> ANIVGGIEYSINNASLCSVGFSVTRGATKGFVTAGHCGTVNATARIGGAVVGTFAARVFPGNDRAWVSLTSAQTLLPRVANGSSFVTVRGSTEAAVGAAVCRSGRTTGYQCGTITAKNVTANYAEGAVRGLTQGNACMGRGDSGGSWITSAGQAQGVMSGGNVQSNGNNCGIPASQRSSLFERLQPILSQYGLSL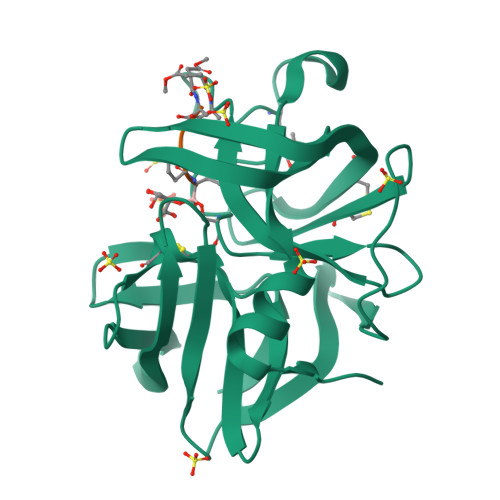VTG;> XAAPV>[2x]MSHKVTKAHNGATLTVAVGELVEIQLPSNPTTG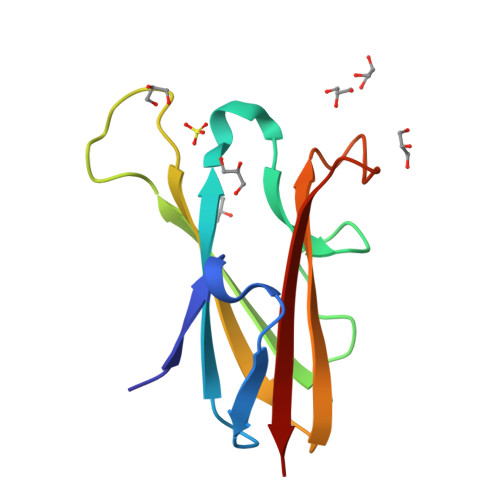FAWYFEGGTKESPNESMFTVENKYFPPDSKLLGAGGTEHFHVTVKAAGTHAVNLTYMRPWTGPSHDSERFTVYLKAN>[4x]GSHMASMYDLIIIGGGPAGLTAGIYAVRYGLDTLILERNEISGQISMADIVENYPGFPSISGLELMERFRTHAQEVGVKTTITEVLSVRSEGTKKIITTDSGDLEAKAVIIATGANPKHLGVPGEKELISKGVSYCAICDGPFFRNKIVAVVGGGNSAVTDALFLSKVA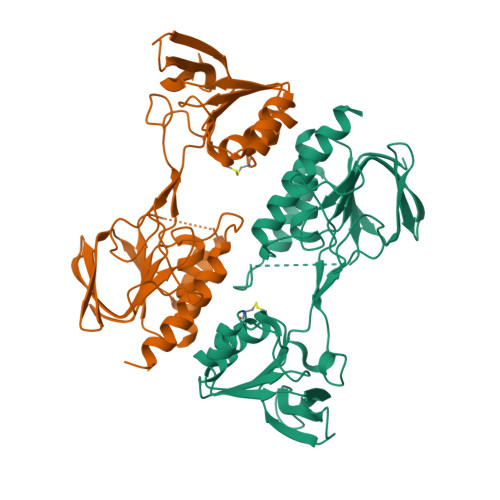QKVYLVHRRDHLKAARVLQDRVDGTPNIELILNSHVLEIVGTREGIKKVEKIILEDVNSRETRELSTNGVFIYVGIHPNTEFVDVEKDEGGFIKTDRWMETSEKGIYAAGDCRDTPIWQLVTAVRDGAIAATAAYEYIEKIR> SPKGTGASTE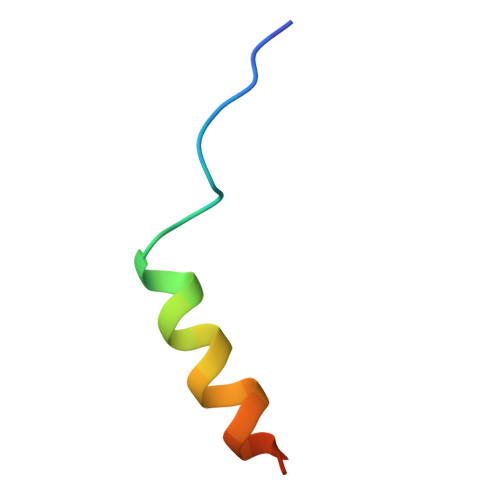VKQKLQEFLLSKSATK> QKPYKETYGISHITRHDMLQIPEQQKNEKYQVPEFDSSTIKNISSAKGLDVWDSWPLQNADGTVANYHGYH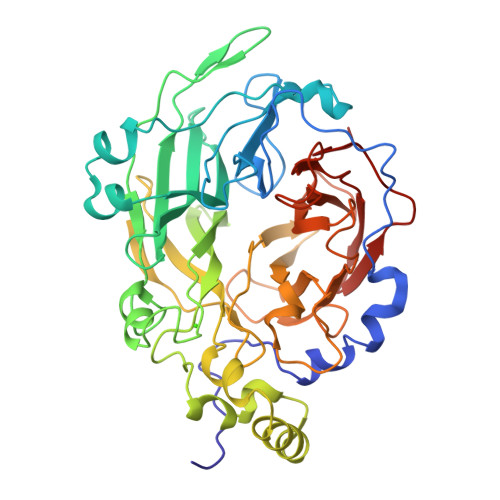IVFALAGDPKNADDTSIYMFYQKVGETSIDSWKNAGRVFKDSDKFDANDSILKDQTQEWAGSATFTSDGKIRLFYTDFSGKHYGKQTLTTAQVNVSASDSSLNINGVEDYKSIFDGDGKTYQNVQQFIDEGNYSSGDNHTLRDPHYVEDKGHKYLVFEANTGTEDGYQGEESLFNKAYYGKSTSFFRQESQKLLQSDKKRTAELANGALGMIELNDDYTLKKVMKPLIASNTVTDEIERANVFKMNGKWYLFTDSRGSKMTIDGITSNDIYMLGYVSNSLTGPYKPLNKTGLVLKMDLDPNDVTFTYSHFAVPQAKGNNVVITSYMTNRGFYADKQSTFAPSFLLNIKGKKTSVVKDSILEQGQLTVN> GSFTMEPLKVEKFATANRGNGLRAVTPLRPGELLFRSDPLAYTVCKGSRGVVCDRCLLGKEKLMRCSQCRVAKYCSAKCQKKAWPDHKRECKCLKSCKPRYPPDSVRLLGRVVFKLMDGAPSESEKLYSFYDLESNINKLTEDKKEGLRQLVMTFQHFMREEIQDASQLPPAFDLFEAFAKVICNSFTICNAEMQEVGVGLYPSISLLNHSCDPNCSIVFNGPHLLLRAVRDIEVGEELTICYLDMLMTSEERRKQLRDQYCFECDCFRCQTQDKDADMLTGDEQVWKEVQESLKKIEELKAHWKWEQVLAMCQAIISSNSERLPDINIYQLKVLDCAMDACINLGLLEEALFYGTRTMEPYRIFFPGSHPVRGVQVMKVGKLQLHQGMFPQAMKN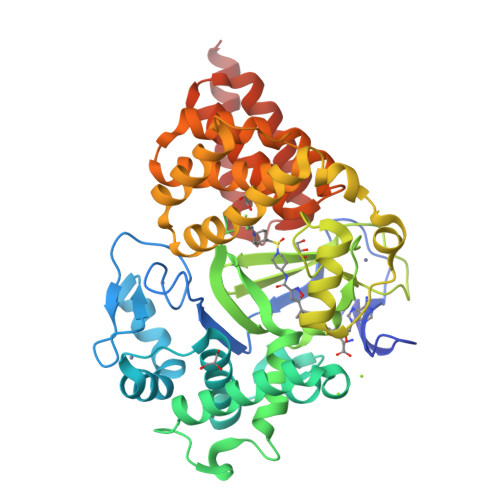LRLAFDIMRVTHGREHSLIEDLILLLEECDANIRAS>SNVPHKSSLPEGIRPGTVLRIRGLVPPNASRFHVNLLCGEEQGSDAALHFNPRLDTSE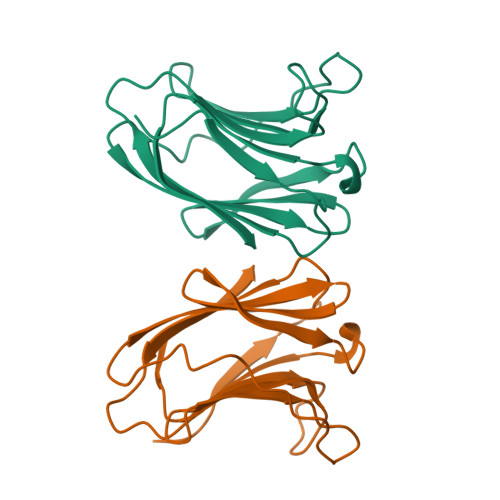VVFNSKEQGSWGREERGPGVPFQRGQPFEVLIIASDDGFKAVVGDAQYHHFRHRLPLARVRLVEVGGDVQLDSVRIF[2x]>[2x]MSNFEKRNRKMAEKNIRKPKQERSIEKRNKILQVAKDLFSDKTYFNVTTN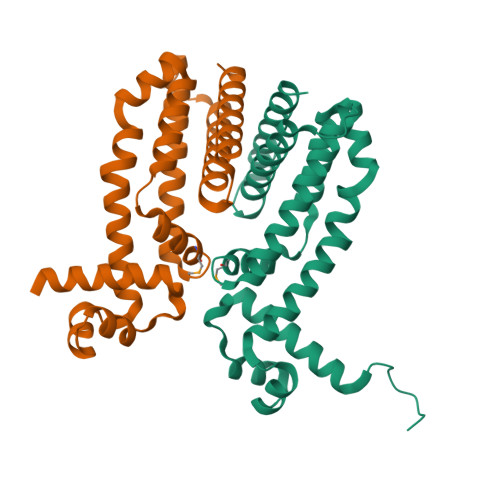EIAKKADVSVGTLYAYFASKEDILTALLKRYNDFFLTTIFADINSQDSLDRFKKNPKEWLNVLINQLLAAEDKIFHAQIEMLAYAIPQAKALLEEHNNNLKNLTYKCLLYYSDQAANPSFKTLSLVVFDFISALVDELLYHEHTQEEAHQIKKTGIDSLDLIIKSYL> AQLTIEAVPSNAAEG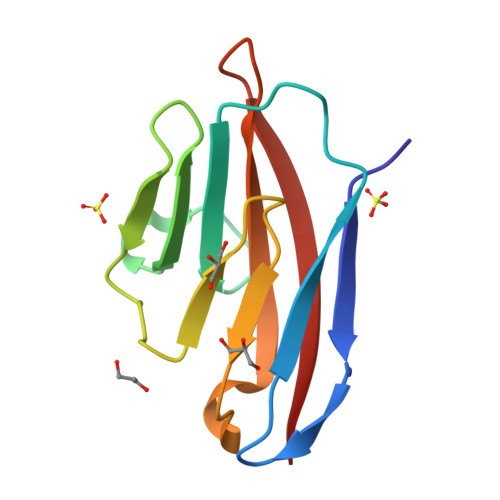KEVLLLVHNLPQDPRGYNWYKGETVDANRRIIGYVISNQQITPGPAYSNRETIYPNASLLMRNVTRNDTGSYTLQVIKLNLMSEEVTGQFSVH>[2x]GMTESDRDQEASMREVVIVKSTPQRGKFNAFAELVGK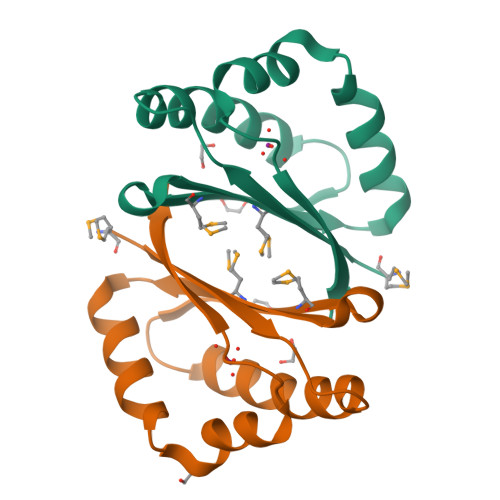LVSETRDFPGCLGAYLMLAPERNEQVVMHIWETPDALEAYLTWRADRGDFLEINEYLEVEQDFKTYQLA>MTKRVAVIGAGPSGLAQLRAFQSAADQGAEIPEIVCFEKQANWGGLWNYTWRTGLDENGEPVHCSMYRYLWSNGPKEGLEFADYSFEEHFGKQIASYPPRAVLFDYIEGRVHKADVRKWIRFNSPVRWVSYDAETAKFTVTAHNHETDSTYSAAFDHVICASGHFSTPNVPFYEGFDTFNGRIVHAHDFRDAREFEGKDVLVMGASYSAEDIGSQCWKYGAKSITSCYRSAPMGYAWPDNWEEKPALEKLTGKTAHFADGSTRDVDAIILCTGYKHFFSFLPDDLRLKTANRLATADLYKGVAYVHNPAMFYLGMQDQ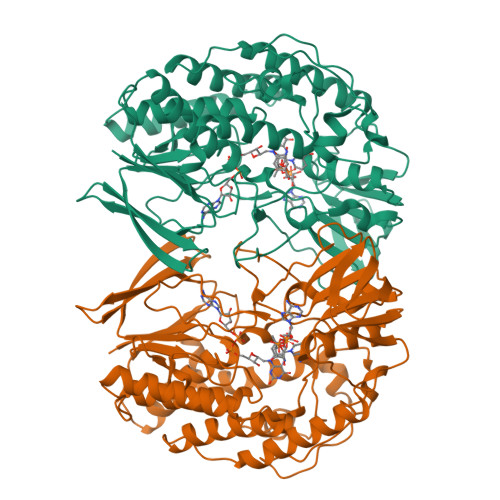WFTFNMFDAQAWWVRDAILGRITLPKDKAAMLADVAERETREEASDDVKYAIRYQADYVKELVAETDYPSFDIDGACDAFFEWKKHKAKDIMAFRDNSYKSVITGTMAPVHHTPWKEALDDSMEAYLQNHHHHHH[2x]> MLVI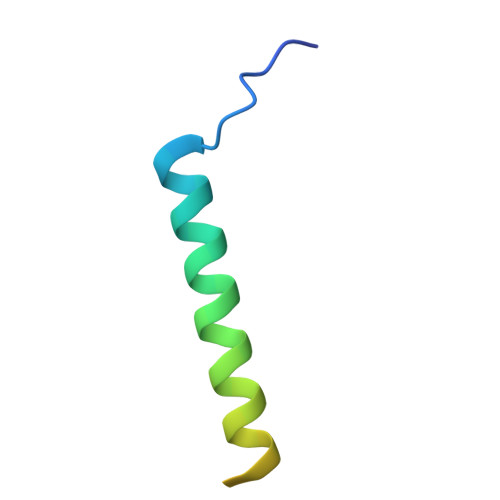PPGMSEEEEALQKKFMKLKKKKKALMALKKQSSSSTTSQGGVKRSLY> MTLTYWDKEKRMTLKQMIQQVAINEQENELTHYVFTTPLSMPTFGKPMLGYVPLNEV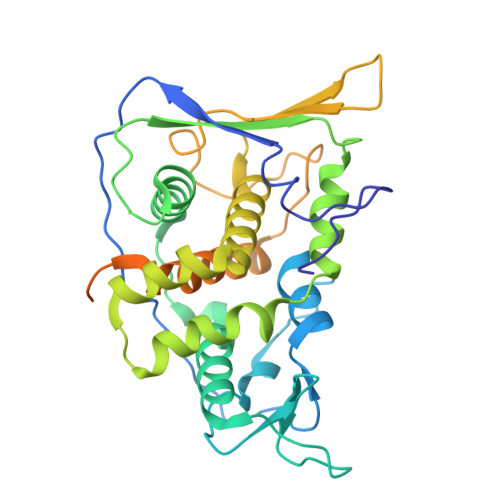ATSKFFSNVNDFDRDNQLAMAHFPDTTITQAYNLTNSIKPGDTSLPDAEVAALKWFWKFFTSINLVRQPPMDNVMYWACQFLSSGTSFLPLERDVEIVFSGFKGSHICMFSNLRQMNLSPILCPYYDLITNFKTTTEIRAYVDAHEELKSLLTYLCLCTIVGLCDTFTETRNMDTGEYVWKVRDVVSRNHTPAQNVEKFCYTIQNAKYMIQLVHVLLFPLTDNKYADLPNYVAVITQGAINQSRSHNVINTTDESNSNTTSDTAASTSGIVSGDTGTVASLYPDEFKYVQS> MLKRVEIFTDGSCLGNPGPGGYGAILRYRGREKTFSAGYTRTTNNRMELMAAIVALEALKEHCEVILSTDSQYVRQGITQWIHNWKKRGWKKADKKPVKNVDLWKRLDAALGRHKIKWEWVKGHAG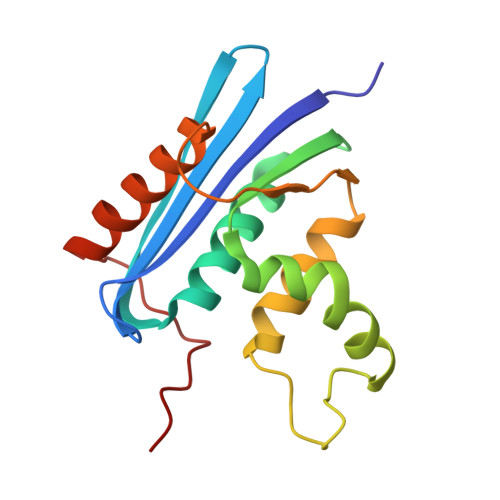HPENERCDELARAAAMKPKLEDTGYQVEV> IVGGQECKDGECPWQALLINEENEGFCGGTILSEFYILTAAHCLYQAKRF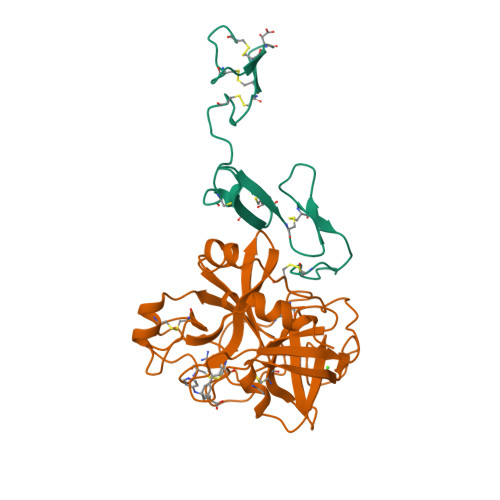KVRVGDRNTEQEEGGEAVHEVEVVIKHNRFTKETYDFDIAVLRLKTPITFRMNVAPACLPERDWAESTLMTQKTGIVSGFGRTHEKGRQSTRLKMLEVPYVDRNSCKLSSSFIITQNMFCAGYDTKQEDACQGDSGGPHVTRFKDTYFVTGIVSWGEGCARKGKYGIYTKVTAFLKWIDRSMKTR;> KDGDQCETSPCQNQGKCKDGLGEYTCTCLEGFEGKNCELFTRKLCSLDNGDCDQFCHEEQNSVVCSCARGYTLADNGKACIPTGPYPCGKQTLER> MGSSHHHHHHENLYFQGGYVIMTKTNGRNAQIKDTFNQTLKLYPTKNLDDFYDKEGFRDQEFKKGDKGTWIVNSEMVIEPKGKDMETRGMVLYINRNTRTTKGYYFISEMTDDSNGRPKDDEKRYPVKMEHNKIIPTKPLPNDKLKKE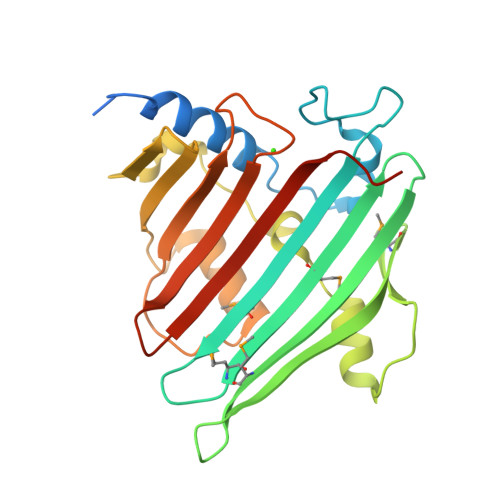IENFKFFVQYGNFKDINDYKDGDISYNPNVPSYSAKYQLNNDDYNVQQLRKRYDIPTKQAPKLLLKGDGDLKGSSVGSRSLEFTFVENKEENIYFTDSVQYTPSEDTRYESN>[2x]MHHHHHHHHHHSSGVDLGTENLYFQSNAMKTLEKVNYKGFIWPLAVGIVLWLITPWRPGGLSVQAWEMFAIFVATIVGCITKPLPIGGTTLLGMVVTVLVGLAPVKDVVNSKGVVIQTGILSSFGNSAAWLIAMAFIMAHGISKTGLGNRVAYVMIEKFGKRSIGIGY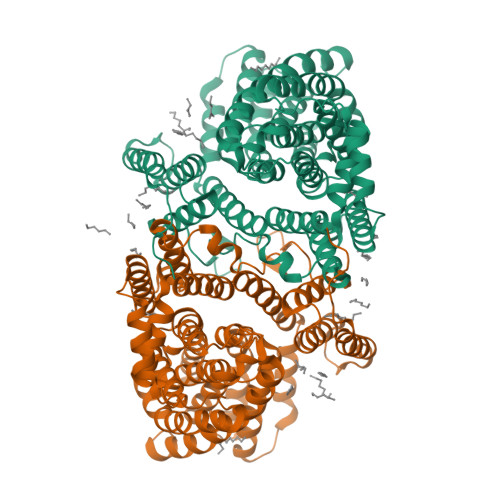AITGLELMMGALIPSNSARTGGVTWPVVESISKSYDSKPNDPSRKKIGAYLDFMAFHANILSTALFITGAAPNLVAQQMAAQKGYQMSWVSWFWAALVPVLVATVIIPLVIYKMYPPEVKETPNAKNWADDKLKEMGPISKPEKIMATVFCLAILLWVLSGFFKIPQLDSAFVAFLAVTLLLITGVLSMEDALHETGAWNILIWLSILIFMAGKLISYGFIAWFAKFIQSEVHGINWGLVLVVLILLMFYTHYFFASGTAHMTALYLPFLTVATAMGAPLGLSAMLLAFTGVINASTTHYANGPASILATTGYVKQSEWWKMNFILGLIYMVIFGIVGTIWMKIIGIW> MATIRPDDKAIDAAARHYGITLDKTAR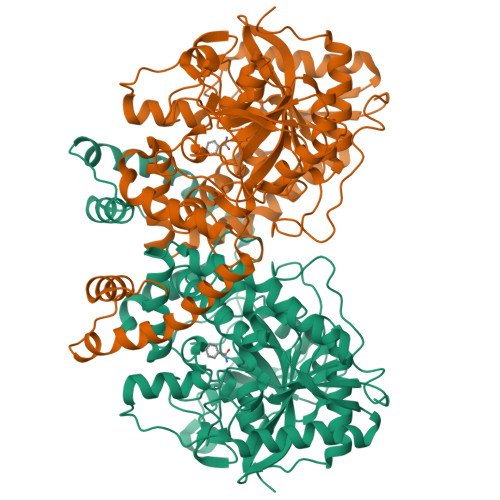LEWPALIDGALGSYDVVDQLYADEATPPTTSREHAVPSASENPLSAWYVTTSIPPTSDGVLTGRRVAIKDNVTVAGVPMMNGSRTVEGFTPSRDATVVTRLLAAGATVAGKAVCEDLCFSGSSFTPASGPVRNPWDRQREAGGSSGGSAALVANGDVDFAIGGDQGGAIRIPAAFCGVVGHKPTFGLVPYTGAFPIERTIDHLGPITRTVHDAALMLSVIAGRDGNDPRQADSVEAGDYLSTLDSDVDGLRIGIVREGFGHAVSQPEVDDAVRAAAHSLTEIGCTVEEVNIPWHLHAFHIWNVIATDGGAYQMLDGNGYGMNAEGLYDPELMAHFASRRIQHADALSETVKLVALTGHHGITTLGGASYGKARNLVPLARAAYDTALRQFDVLVMPTLPYVASELPAKDVDRATFITKALGMIANTAPFDVTGHPSLSVPAGLVNGLPVGMMITGRHFDDATVLRVGRAFEKLRGAFPTPAERASNSAPQLSPA4-[3,6-bis(chloranyl)-2-fluoranyl-phenyl]carbonyl-~{N}-(1-methylpyrazol-4-yl)-1~{H}-pyrrole-2-carboxamide | C16 H11 Cl2 F N4 O2 | 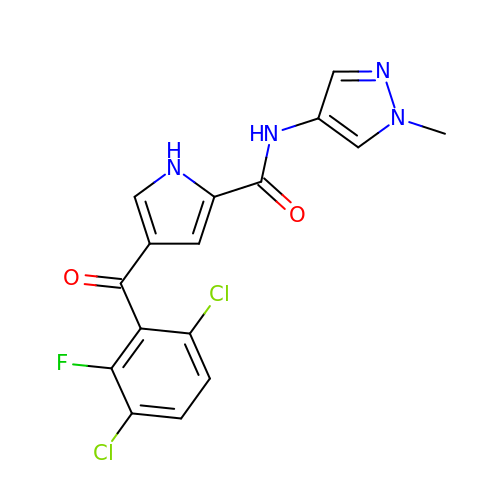LIEUQFMVFKJKHX-UHFFFAOYSA-N> GPLGSECPDRWRAEIDLGLPPGVQVGDLLRNEQTMGSLRQVYLLAVQANSITDHLKRFDAVRVP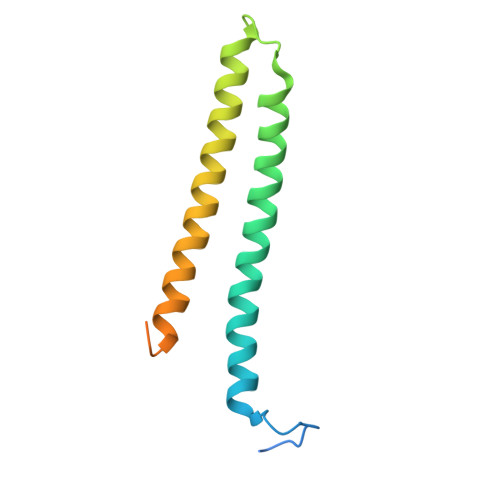ESCRGVVEAQVAKLEAVRSVIWNTMISLAVSGIEMDENGLKALLDKQAGDSLALMEMEKVATALKMD> NAAYYQVVPVTANVYDSDGEKLSYISQGSVVWLDKDRKSDDKRLAITISGLSGYMKTEDLQALDASKDFIPYYESDG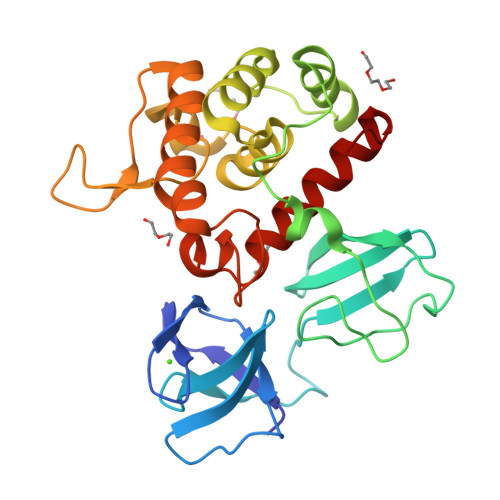HRFYHYVAQNASIPVASHLSDMEVGKKYYSADGLHFDGFKLENPFLFKDLTEATNYSAEELDKVFSLLNINNSLLENKGATFKEAEEHYHINALYLLAHSALESNWGRSKIAKDKNNFFGITAYDTTPYLSAKTFDDVDKGILGATKWIKENYIDRGRTFLGNKASGMNVEYASDPYWGEKIASVMMKINEKLGGKD> MSMMAERDMGRILLDLSDDVIQRLDDLKVQRNIPRAELLREAVEQYLEKQDRAKDTISSALGLWQD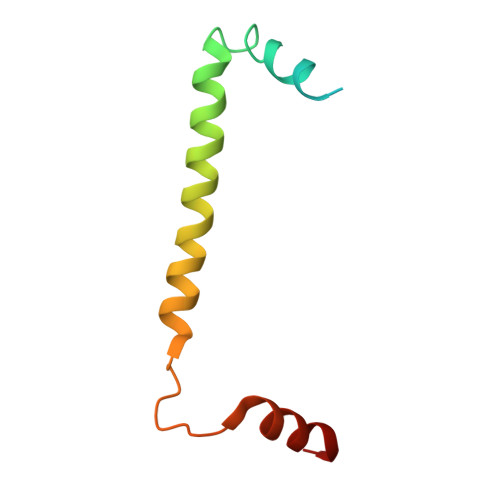CEEDGMEYQRQLRKEW>MVRKGAAAKAPQQPKPKAQQQPGGR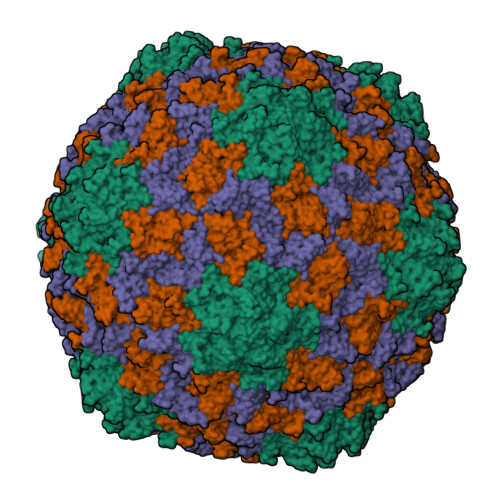RRRRGRSMEPVSRPLNPPAAVGSTLKAGRGRTAGVSDWFDTGMITSYLGGFQRTAGTTDSQVFIVSPAALDRVGTIAKAYALWRPKHWEIVYLPRCSTQTDGSIEMGFLLDYADSVPTNTRTMASSTSFTTSNVWGGGDGSSLLHTSMKSMGNAVTSALPCDEFSNKWFKLSWSTPEESENAHLTDTYVPARFVVRSDFPVVTADQPGHLWLRSRILLKGSVSPSTNL[3x]>[3x]PIATPYPVKEWLQPKRYKAHLMGTTYVYDFPELFRQASSSQWKNFSADVKLTDDFFISNELIEDENGELTEVEREPGANAIGMVAFKITVKTPEYPRGRQFVVVANDITFKIGSFGPQEDEFFNKVTEYARKRGIPRIYLAANSGARIGMAEEIVPLFQVAWNDAANPDKGFQYLYLTSEGMETLKKFDKENSVLTERTVINGEERFVIKTIIGSEDGLGVECLRGSGLIAGATSRAYHDIFTITLVTCRSVGIGAYLVRLGQRAIQVEGQPIILTGAPAINKMLGREVYTSNLQLGGTQIMYNNGVSHLTAVDDLAGVEKIVEWMSYVPAKRNMPVPILETKDTWDRPVDFTPTNDETYDVRWMIEGRETESGFEYGLFDKGSFFETLSGWAKGVVVGRARLGGIPLGVIGVETRTVENLIPADPANPNSAETLIQE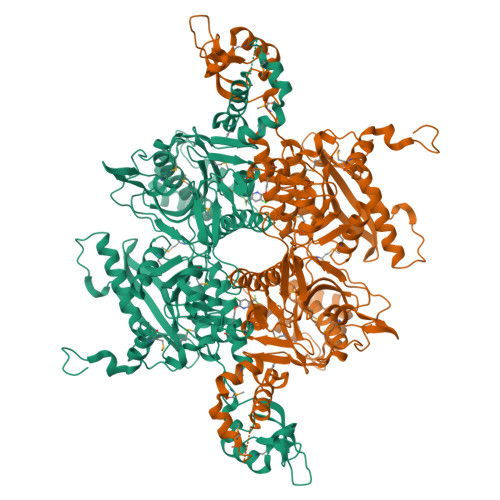PGQVWHPNSAFKTAQAINDFNNGEQLPMMILANWRGFSGGQRDMFNEVLKYGSFIVDALVDYKQPIIIYIPPTGELRGGSWVVVDPTINADQMEMYADVNARAGVLEPQGMVGIKFRREKLLDTMNRLDDKYRELRSQLSNKSLAPEVHQQISKQLADRERELLPIYGQISLQFADLHDRSSRMVAKGVISKELEWTEARRFFFWRLRRRLNEEYLIKRLSHQVGEASRLEKIARIRSWYPASVDHEDDRQVATWIEENYKTLDDKLKGLKLESFAQDLAKKIRSDHDNAIDGLSEVIK> MAHAGRTGYDNREIVMKYIHYKLSQRGYEWDAGDDVEENRTEAPEGTESEVVHLTLRQAGDDFSRRYRRDFAEMSSQLHLTPFTARGRFAT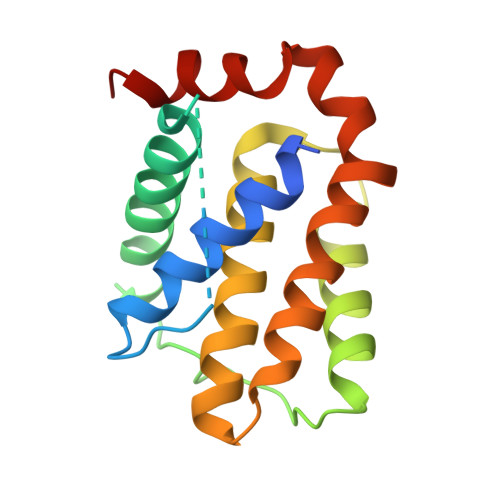VVEELFRDGVNWGRIVAFFEFGGVMCVESVNREMSPLVDNIALWMTEYLNRHLHTWIQDNGGWDAFVELYGPSMR>[2x]MGHHHHHMVLADLGRKITSALRSLSNATIINEEVLNAMLKEVCTALLEADVNIKLVKQLRENVKSAIDLEEMASGLNKRKMIQHAVFKELVKLVDPGVKAWTPTKGKQNVIMFVGLQGSGKTTTCSKLAYYYQRKGWKTCLICADTFRAGAFDQLKQNATKARIPFYGSYTEMDPVIIASEGVEKFKNENFEIIIVDTSGRHKQEDSLFEEMLQVANAIQPDNIVYVMDA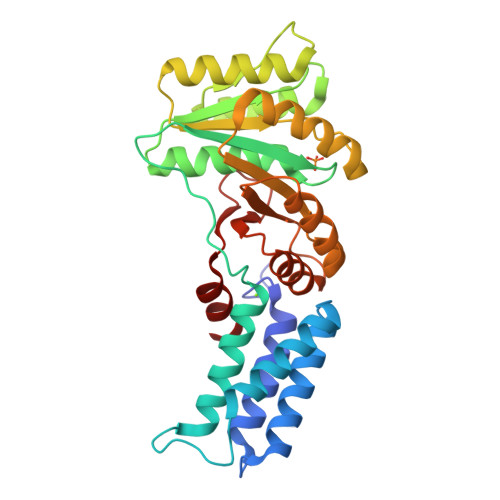SIGQACEAQAKAFKDKVDVASVIVTKLDGHAKGGGALSAVAATKSPIIFIGTGEHIDDFEPFKTQPFISKLLG>MSLAARLIRSSRSNTFGIITDYVSTTPYSVDIVRGIQDW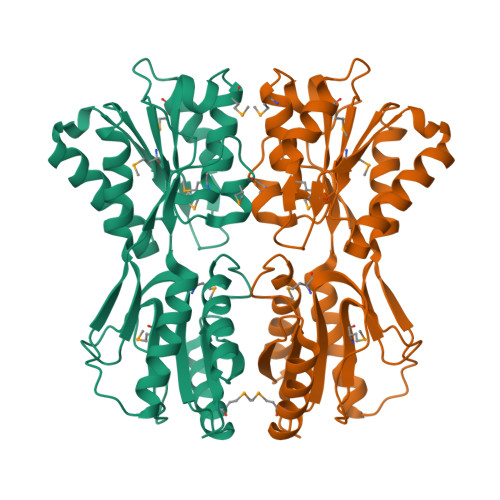ANANGKTILIANTGGSSEREVEIWKMFQSHRIDGVLYVTMYRRIVDPESGDVSIPTVMINCRPQTRELLPSIEPDDYQGARDLTRYLLERGHRRIGYIRLNPILLGAELRLDAFRRTTSEFGLTENDLSISLGMDGPVGAENNYVFAAATEMLKQDDRPTAIMSGNDEMAIQIYIAAMALGLRIPQDVSIVGFDDFRTVTMALKPELTTAALPYYDLGREGAKWLNDLIAGEKIYPGSRVVSCKLVERSSAAFGEGHHHHHH[2x]The FimA subunits of the pilus rod are single domain proteins of 16 kDa with an incomplete, immunoglobulin (IG)2-like fold that lacks the C-terminal β-strand (G-strand). In the structure of the pilus rod, the FimA subunits interact via inter-molecular donor strand complementation, in which the N-terminal extension of each subunit, termed the donor strand, inserts as a β-strand into the preceding subunit and completes its IG-like fold. In 2010, Sukumaran et al. discovered that the FimA proteins from the enteroinvasive pathogens E. coli, Shigella flexneri, and Salmonella enterica have a second function besides formation of homopolymeric pilus rods; soluble forms of FimA, independent of FimC, act as inhibitors of host cell apoptosis after pathogen internalization by stabilizing the interaction between hexokinase and the voltage-dependent anion channel (VDAC) on the surface of mitochondria. We showed that all three FimA orthologues investigated (FimAECO, FimASHI, and FimASAL) were capable of folding to an alternative, self-complemented, monomeric form of only marginal thermodynamic stability that likely represents the FimA species that acts as an inhibitor of host cell apoptosis after internalization of the respective pathogen.

FimAECO, FimASHI, and FimASAL were produced as reduced, insoluble proteins in the E. coli cytoplasm without their N-terminal signal sequences. All proteins were refolded in the absence of the chaperone FimC under oxidizing conditions to allow the formation of the single, invariant structural disulfide bond. The purified proteins were crystallized, and their X-ray structures were determined at 1.5, 0.89, and 1.69 Å resolution, respectively. All FimA orthologues crystallized as self-complemented monomers, and all structures strongly resembled the previously reported NMR structure of the FimAECO monomer. Specifically, all three FimA monomers showed nearly identical immunoglobulin-like folds, completed by intramolecular donor strand insertion in a parallel orientation relative to the C-terminal F-strand. The global folds and registers of parallel donor strand insertion in the X-ray structures of FimASHI and FimASAL were the same as those observed in FimAECO, and all three structures showed high surface complementarity between donor strand and the rest of the folded FimA domain. The overall pairwise Cα RMSD values for the three X-ray structures were 0.30 Å for FimAECO/FimASHI (113 Cα atoms), 0.51 Å for FimAECO/FimASAL (154 Cα atoms), and 0.57 Å for FimASAL/FimASHI (110 Cα atoms), and the only minor conformational differences were restricted to loop segments 15–20, 37–45, and 89–97, and residues 51 and 81. Evaluation of the data according to the two-state model of folding revealed that all FimA orthologues proved to be only marginally stable, with free energies of folding at zero denaturant (ΔG0) of only −5.5, −8.9, and −7.2 kJ/mol for FimAECO, FimASHI, and FimASAL, respectively.

> MLADTTTVNGGTIHFKGEVVNAACAVDAGSVDQTVQLGQVRTASLKQAGATSSAVGFNIQLNDCDTTVATKAAVAFLGTAIDATRTDVLALQSSAAGSATNVGVQILDRTGNALTLDGATFSAQTTLNNGTNTIPFQARYYAIGEATPGAANADATFKVQYQ> QSPPGKPEIHKCRSPDKETFTCWWNPGTDGGLPTNYSLTYSKEGEKTTYECPDYKTSGPNSCFFSKQYTSIWKIYIITVNATNQMGSSSSDPLYVDVTYIVEPE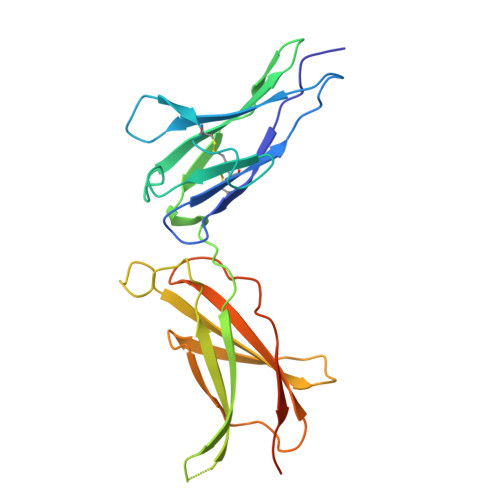PPRNLTLEVKQLKDKKTYLWVKWSPPTITDVKTGWFTMEYEIRLKPEEAEEWEIHFTGHQTQFKVFDLYPGQKYLVQTRCKPDHGYWSRWSQESSVEMPNDFTLKDRSRSHHHHHH> MKTSSNASITDGNGNYSIAGATYGVFADKDCTKQLATLTTNENGNTDVVEVTTGTVYIRELSAPAGYKVDKTVYSLKVEA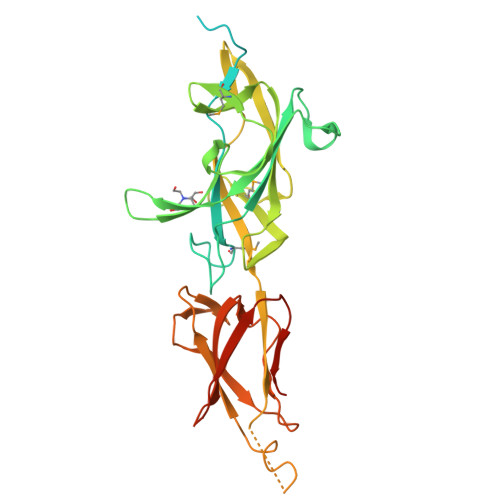GKTATLKVSDTPKVTDTLIELFKIDMETQKDNPQGNASLAGAEFTWKYYAGFYNKENLPAEATRTWVTKTIAETDSDGTTHYITKLADAYKVSGDSFYMQDGKAVLPLGTLTVEETKAPNGYLLDGAYMQAGDKSEQIKGLYVTQITEDGDLAVLSGSNQFSVSDKVIRGGVKIQKRDLETGDTKPQGSATLKDTAFDIISLNDNVVLVEGKLYKKNEVVKTIHTDIEGVASTSADLLPYGKFRIVESEAPNGYLTDGAKPIDFAITENGKIVDLTDEAHSGAAL> VTNVGEDGEPGETEPRHALSPVDMHVHTDVSFLLDRFFDVETLELSNLTGSPATHVLDPFGSTAQLAWARL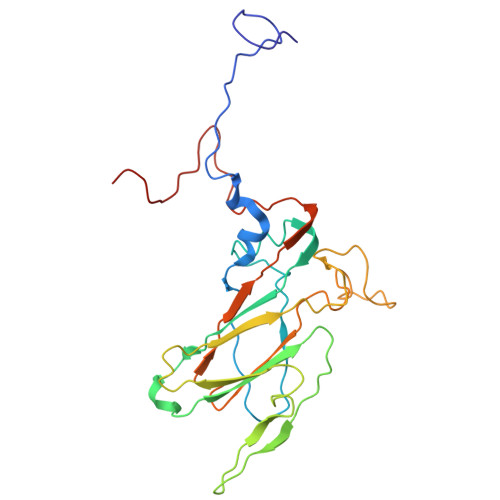LNTCTYFFSDLELSIQFKFTTTPSSVGEGFVWVKWFPVGAPTKTTDAWQLEGGGNSVRIQQLAVAGMSPTVVFKIAGSRSQACGFSVPYTSMWRVVPVFYNGWGAPTKEKATYNWLPGAHFGSILLTSDAHDKGGCYLRYRFPRANMYCPRPIPPAFTRPADKTRHKFPTNINKQCT> ACDY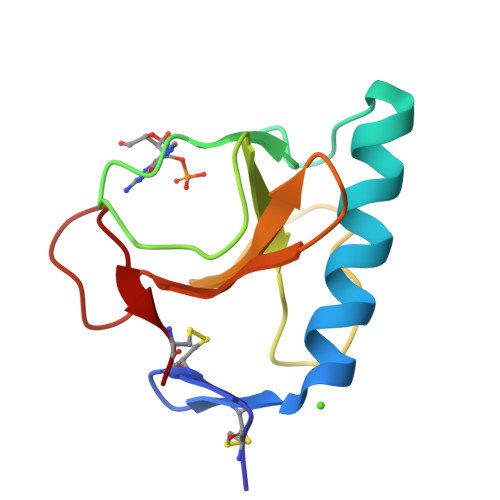TCGSNCYSSSDASTAQAAGYKLHEDGETVGSNSYPHKYNNYEGFDFSVSSPYYEWPILSSGDVYSGGSPGADRVVFNENNQLAGVITHTGASGNNFVECT> WEHRRFIVADSRNFITPEFPRDFWMSPV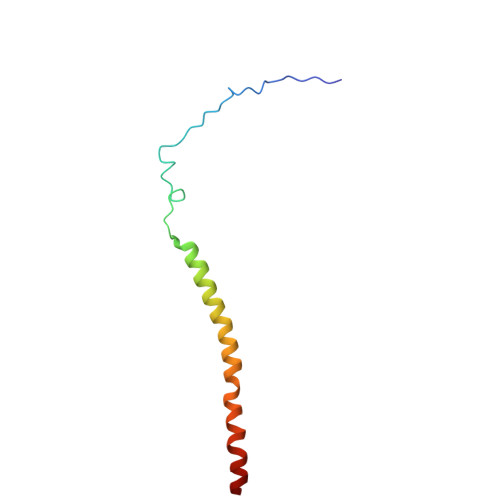FNLPRETAAEQVVVLQAQRTAAAAALENAAMQAAELPVDIERRLRPIERNVH> VIHYSSGKDLCPVKGWAPLSKDNGIRIGSRGEVFVIREPFISCSINECRTFFLTQGALLNDKHSNGTVKDRSPFRTLMSCPIGVAPSPSNSRFESVAWSATACSDGPGWLTIGITGPDATAVAVLKYNGIITDTLKSWKGNIMRTQESECVCQDEFCYTLITDGPSDAQAFYKILKIKKGKIVSVKDVDAPGFHFEECSCYPSGENVECVCRDNWRGSNRPWIRFNSDLDYQIGYVCSGVFGDNPRPMDSTGSCNSPINNGKGRYGVKGFSFRYGDGVWIGRTKSLESRSGFEMVWDANGWVSTDKDSNGVQDIIDNDN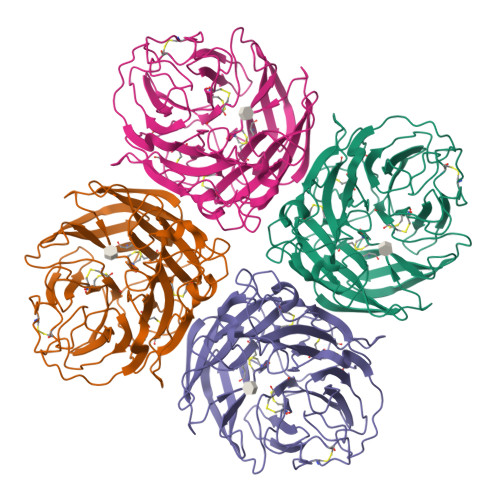WSGYSGSFSIRGETTGRNCTVPCFWVEMIRGQPKEKTIWTSGSSIAFCGVNSDTTGWSWPDGALLPFDIDK> PKRPT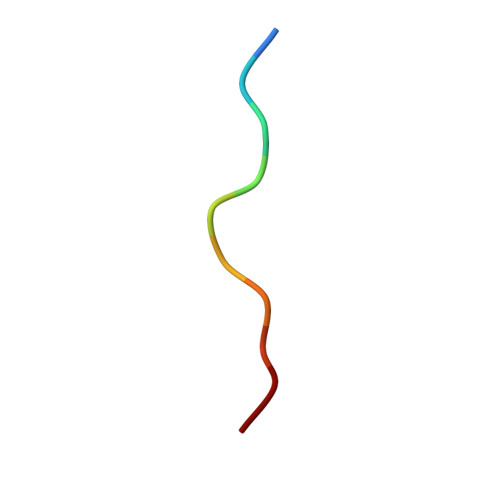TLNLF>MAHTGRMFKIEAAEIVVARLPLKFRFETSFGVQTHKVVPLLILHGEGVQGVAEGTMEARPMYREETIAGALDLLRGTFLPAILGQTFANPEAVSDALGSYRGNRMARAMVEMAAWDLWARTLGVPLGTLLGGHKEQVEVGVSLGIQADEQATVDLVRRHVEQGYRRIKLKIKPGWDVQPVRATREAFPDIRLTVDANSAYTLADAGRLRQLDEYDLTCIEQPLAWDDLVDHAELARRIRTPLCLDESVASASDARKALALGAGGVINLKVARVGGHAESRRVHDVAQSFGAPVWCGGMLESGIGRAHNIHLSTLSNFRLPGDTSSASRYWERDLIQEPLEAVDGLMPVPQGPGTGVTLDREFLATVTEAQEEHR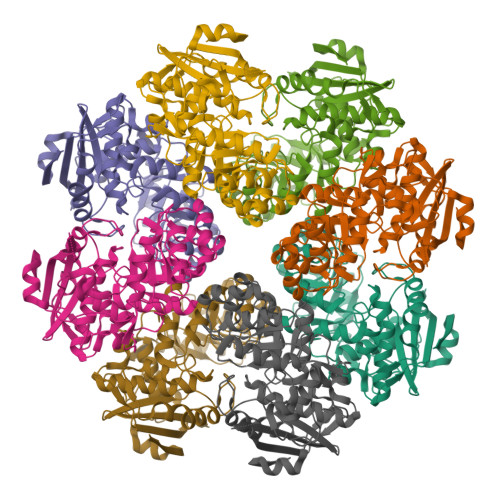A[4x]>[6x]MADVFHLGLTKAMLDGATLAIVPGDPERVKRIAELMDNATFLASHREYTSYLAYADGKPVV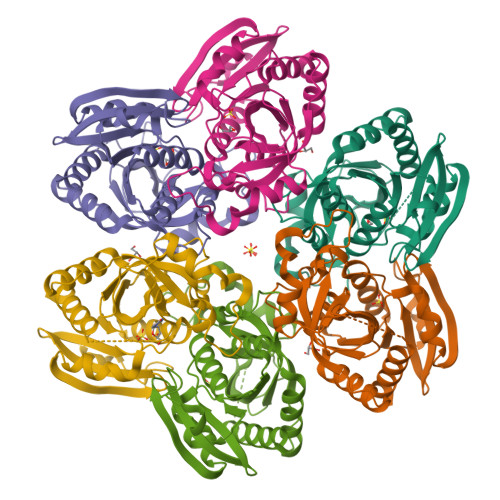ICSTGIGGPSTSIAVEELAQLGVNTFLRVGTTGAIQPHVNVGDVIVTQASVRLDGASLHFAPMEFPAVANFECTTAMVAACRDAGVEPHIGVTASSDTFYPGQERYDTVTGRVTRRFAGSMKEWQDMGVLNYEMESATLFTMCATQGWRAACVAGVIVNRTQQEIPDEATMKKTEVSAVSIVVAAAKKLLA>MGSSHHHHHHSSGLVPRGSHSMKETRDLETLSVNAIRFLAIDAVEKARSGHPGMPMGMAPLAYLLFREVMRHNPLDPDWPDRDRFVLSAGHGSMLLYAVLHLTGYDLPLEELKSFRQWGSKTPGHPERGHTPGVEVTTGPLGQGISTAVGLALAERKLAAEFNRPGHVVVDHYTYVLASDGDLMEGVSGEAASLAGHWGLSKLIVFWDDNRISIDGPTDLAFTEDVLARYRAYGWQTLRVEDVNDLEALRKAIKLAKLDERPTLIAVRSHIGFGSPKQDSAKAHGEPLGPEAVEATRRNLGWPYPPFVVPEEVYRHMDMREKGRAWQEAWEKALEAYARAYPDLHQELMRRLRGELPPLPEEPPSFDKPIATRAASGRALNLLAPRLPELLGGSADLTPSNNTKAEGMEDFSRANPLGRYLHFGVREHAMGAILNGLNLHGGYRAYGGTFLVFSDYMRPAIRLAALMGVPTVFVFTHDSIALGEDGPTHQPVEHLMSLRAMPNLFVIRPADAYETFYAWLVALRRKEGPTALVLTRQAVPLLSPEKARGLLRGGYVLEDVEEPQGVLVATGSEVHLALRAQALLREKGVRVRVVSLPSFELFAAQPEAYRKEVLPPGLPVVAVEAGASLGWERYAHKVVALDR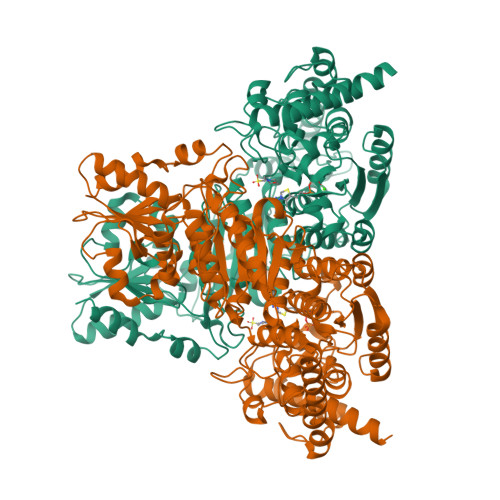FGASAPYPEVYERLGFTPERVAEAFLSLV[4x]>[2x]MILFDKNKRILKKYAKMVSKINQIESDLRSKKNSELIRLSMVLKEKVNSFEDADEHLFEAFALVREAARRTLGMRPFDVQVMGGIALHEGKVAEMKTGEGKTLAATMPIYLNALIGKGVHLVTVNDYLARRDALWMGPVYLFLGLRVGVINSLGKSYEVVWKNPDLARKAIEENWSVWPDGFNGEVLKEESMNKEAVEAFQVELKEITRKEAYLCDVTYGTNNEFGFDYLRDNLVLDYNDKVQRGHFYAIVDEADSVLIDEARTPLIISGPSKESPSVYRRFAQIAKKFVKDKDFTVDEKARTIILTEEGVAKAEKIIGVENLYDPGNVSLLYHLINALKALHLFKKDVDYVVMNGEVIIVDEFTGRLLPGRRYSGGLHQAIEAKEGVPIKEESITYATITFQNYFRMYEKLAGMTGTAKTEESEFVQVYGMEVVVIPTHKPMIRKDHDDLVFRTQKEKYEKIVEEIEKRYKKGQPVLVGTTSIEKSELLSSMLKKKGIPHQVLNAKYHEKEAEIVAKAGQKGMVTIATNMAGRGTDIKLGPGVAELGGLCIIGTERHESRRIDNQLRGRAGRQGDPGESIFFLSLEDDLLRIFGSEQIGKVMNILKIEEGQPIQHPMLSKLIENIQKKVEGINFSIRKTLMEMDDVLDKQRRAVYSLRDQILLEKDYDEYLKDIFEDV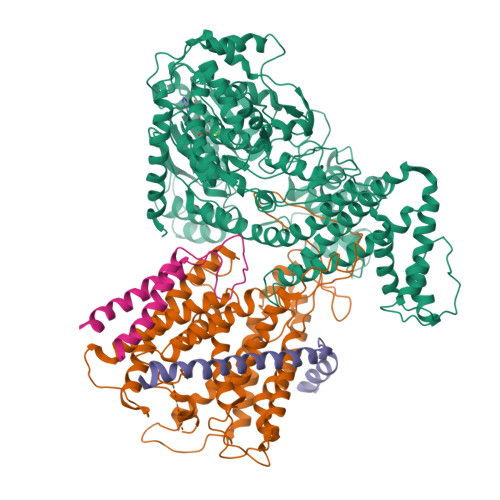VSTRVEEFCSGKNWDIESLKNSLSFFPAGLFDLDEKQFSSSEELHDYLFNRLWEEYQRKKQEIGEDYRKVIRFLMLRIIDDHWRRYLEEVEHVKEAVQLRSYGQKDPIVEFKKETYYMFDEMMRRINDTIANYVLRVVKVSEKDEKEAKEELGKIRLVHEEFNLVNRAMRRATEKKKKKDGLHSFGRIRVKR;>[2x]MWQAFKNAFKIPELRDRIIFTFLALIVFRMGIYIPVPGLNLEAWGEIFRRIAETAGVAGILSFYDVFTGGALSRFSVFTMSVTPYITASIILQLLASVMPSLKEMLREGEEGRKKFAKYTRRLTLLIGGFQAFFVSFSLARSNPDMVAPGVNVLQFTVLSTMSMLAGTMFLLWLGERITEKGIGNGISILIFAGIVARYPSYIRQAYLGGLNLLEWIFLIAVALITIFGIILVQQAERRITIQYARRVTGRRVYGGASTYLPIKVNQGGVIPIIFASAIVSIPSAIASITNNETLKNLFRAGGFLYLLIYGLLVFFFTYFYSVVIFDPREISENIRKYGGYIPGLRPGRSTEQYLHRVLNRVTFIGAVFLVVIALLPYLVQGAIKVNVWIGGTSALIAVGVALDIIQQMETHMVMRHYEGFIKKGKIRGRR;>MEKLRKFFREVIAEAKKISWPSRKELLTSFGVVLVILAVTSVYFFVLDFIFSGVVSAIFKALGIG[2x];>MKTFFLIVHTIISVALIYMVQVQMSKFSELGGAFGSGGLHTVFGRRKGLDTGGKITLVLSVLFFVSCVVTAFVLTR[2x]1-[4-(cyanomethyl)-1-[(3-oxidanyl-4-phenyl-phenyl)methyl]piperidin-4-yl]-3-(cyclopropylcarbonylamino)pyrazole-4-carboxamide 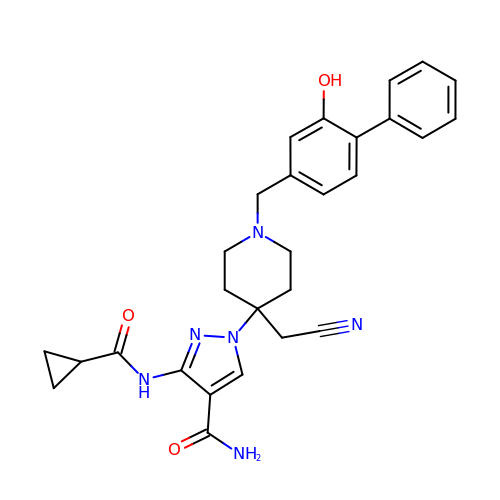| C28 H30 N6 O3 | YQNPSYZTFUVTCR-UHFFFAOYSA-N>[2x]PRVHPARATELTKDAQPSAMDAAGATARPAVRVPQQQAILDPELPAVREPQPPADPEARKVVRGPSHRRGARSTGQPRAPRGSRKEPDKLKKVLDKLRLKRKDISEAAETVNKVVERLLRRMQKRESEFKGVEQLNTGSYYEHVKISAPNEFDV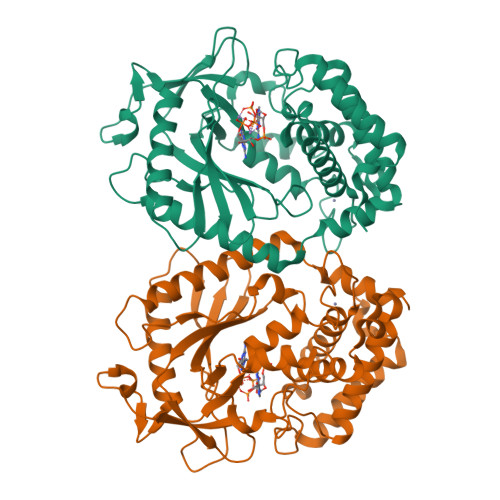MFKLEVPRIELQEYYETGAFYLVKFKRIPRGNPLSHFLEGEVLSATKMLSKFRKIIKEEVKEIKDIDVSVEKEKPGSPAVTLLIRNPEEISVDIILALESKGSWPISTKEGLPIQGWLGTKVRTNLRREPFYLVPKNAKDGNSFQGETWRLSFSHTEKYILNNHGIEKTCCESSGAKCCRKECLKLMKYLLEQLKKEFQELDAFCSYHVKTAIFHMWTQDPQDSQWDPRNLSSCFDKLLAFFLECLRTEKLDHYFIPKFNLFSQELIDRKSKEFLSKKIEYERNNGFPIFDKL The MlaFEDB complex is an ATP-binding cassette transporter to actively translocate the phospholipids between the inner membrane and the periplasmic protein MlaC4,5. The MlaFEDB-mediated glycerophospholipid (PL) transport was reported to play an important role in maintaining the integrity of the lipid membrane. Consistent with the previous reported low-resolution A. baumannii MlaFEDB map8 and our E. coli MlaFEDB map9 (EMD-30355), the MlaF (cytoplasmic nucleotide-binding domain, NBD), MlaE (transmembrane domain), MlaD (periplasmic phospholipid-binding domain), and MlaB (cytoplasmic auxiliary domain) subunits are assembled in a stoichiometry of 2:2:6:2. In summary, we characterize four structures of the A. baumannii MlaFEDB complex in nucleotide-free and vanadate-trapped conformations using single-particle cryo-EM.

To understand the mechanism of glycerophospholipid translocation coupled with the conformational change, distinct conformations of MlaFEDB were trapped using sodium ortho-vanadate. Vanadate acts as a potent inhibitor of ATPase by forming an ADP–vanadate complex that mimics the intermediate state formed during hydrolysis. Three individual conformations were classified and refined to 4.0, 3.6, and 4.0 Å, and were named Vtrans1, Vtrans2, and Vclose, respectively. All three structures display bound nucleotides at the ATP-binding sites. However, the maps are of insufficient quality to distinguish between ADP, ATP, and ADP–vanadate. Comparison of Vtrans1 and Vtrans2 to nucleotide-free structure shows the conformational rearrangement of the MlaD. MlaD hexametric ring rotates clockwise at different levels, whereas MlaFEB remains unchanged. The three vanadate-trapped structures of MlaFEDB reveal different levels of conformational rearrangement of MlaD and MlaE coupled with nucleotide binding and glycerophospholipid translocation.

>[2x]MNTIAWLGRLVIERIRGIGVAALMLLQIIFSLPSAGGFGRFVYQMHRVGVMSLLIITVSGLFIGLVLGLQGYSILVNVGSESMLGTMVSLTLLRELAPVVAALLFAGRAGSALTAEIGSMKQSEQLASMEMIGVDPLKQIVSPRLWAGIVSLPMLTVIFAAIGIVGGKLVGVDFLGVDEGSFWSGMQNNVQFGHDVVNGIIKSIVFALLCTWIAVFQGYACDPTPEGIATAMTRTVVYSSLCVLGFDFVLTAVMFGGI;>MMNNKTPLSTQSLIEVKNLSFNRGERVIYDNISLNIRRGQITAIMGPSGTGKTTLLRLIGGQLVPDQGEVLLDGKDIAQMSRQELFAARARMGMLFQSGALFTDMSVYENVAFPIRAHTKLSENLIAELVALKLESVGLRGTEQLMPTELSGGMNRRVALARAIALDPDLIMYDEPFAGQDPIVKGVLTRLIRSLREALDLTTIIVSHDVPETLSIADYIYVVAEGKIQGEGTPEELQAYASPFVKQFLTGSAEGPVEYQFSHQAYLDNEVRP[2x];>VVQYLNQELVVSGKIDFENAEQQYQAGLAIIKKQTSFPLIVDLKQLEHGNTLALAVLVQWLRQTPQKSGLHFKNVPEKMLKIIQACHLQEDLHLVLEHHHHHH[2x];>[6x]MKSRTSELAVGIFVIIFGIALFFLAMKVSGLVGTNLSDGYTMKAQFDNVNGLKPRAKVTMSGVTIGRVDSITLDPVTRLATVTFDLDGKLTSFNAEQLKEVQKNALDELRYSSDYTQATPAQQKTMEQQLISNMNSITSIDEDAYIMVATNGLLGEKYLKIVPGGGLNYLKRGDTISNTQGTMDLEDLISKFITGGGAGKVAAGSSSAEEKAPASTDSSAQP>MANSITADEIREQFSQAMSAMYQQEVPQYGTLLELVADVNLAVLENNPQLHEKMVNADELARLNVERHGAIRVGTAQELATLRRMFAIMGMYPVSYYDLSQAGVPVHSTAFRPIDDASLARNPFRVFTSLLRLELIENEILRQKAAEILRQRDIFTPRCRQLLEEYEQQGGFNETQAQEFVQEALETFRWHQLATVDEETYRALHNEHRLIADVVCFPGCHINHLTPRTLDIDRVQSMMPECGIEPKILIEGPPRREVPILLRQTSFKALEETVLFAGQKQGTHTA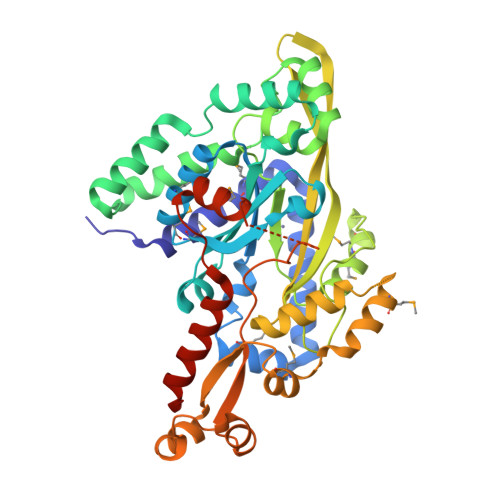RFGEIEQRGVALTPKGRQLYDDLLRNAGTGQDNLTHQMHLQETFRTFPDSEFLMRQQGLAWFRYRLTPSGEAHRQAIHPGDDPQPLIERGWVVAQPITYEDFLPVSAAGIFQSNLGNETQTRSHGNASREAFEQALGCPVLDEFQLYQEAEERSKRRCGLLLEHHHHHH[4x]>MEFTTGLMSLDTALNEMLSRVTPLTAQETLPLVQCFGRILASDVVSPLDVPGFDNSAMDGYAVRLADIASGQPLPVAGKSFAGQPYHGEWPAGTCIRIMTGAPVPEGCEAVVMQEQTEQMDNGVRFTAEVRSGQNIRRRGEDISAGAVVFPAGTRLTTAELPVIASLGIAEVPVIRKVRVALFSTGDELQLPGQPLGDGQIYDTNRLAVHLMLEQLGCEVINLGIIRADPHALRAAFIEADSQADVVISSGGVSVGEADYTKTILEELGEIAFW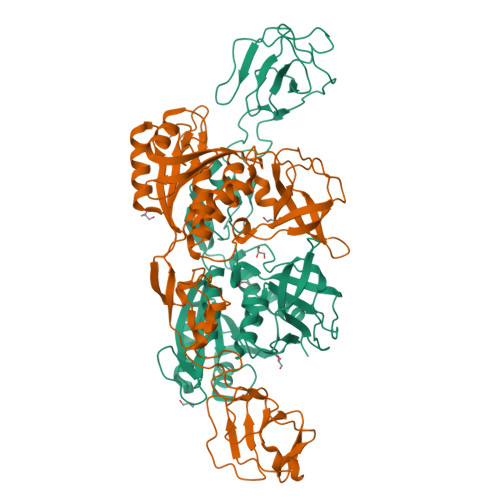KLAIKPGKPFAFGKLSNSWFCGLPGNPVSATLTFYQLVQPLLAKLSGNTASGLPARQRVRTASRLKKTPGRLDFQRGVLQRNADGELEVTTTGHQGSHIFSSFSLGNCFIVLERDRGNVEVGEWVEVEPFNALFGGL[2x]> TSQKHRDFVAEPMGEKPVGSLAGIGEVLGKKL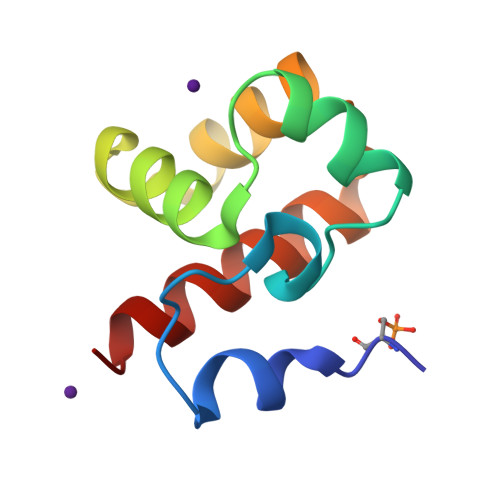EERGFDKAYVVLGQFLVLKKDEDLFREWLKDTAGANAKQSRDAFGALREWADAF>[2x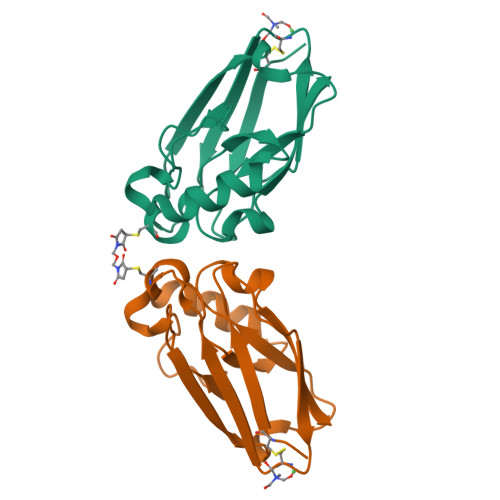]AECSVDIQGNDQMQFNTNAITVDKSCKQFTVNLSHPGNLPKCVMGHNWVLSTAADMQGVVTDGMASGLDKDYLKPDDSRVIAHTKLIGSGEKDSVTFDVSKLKEGEQYMFFCTFPGHSALMKGTLTLK> MSGTLVQRLKLILSGGNLRCSDGETACDPERPPTRCVFQVHGQDGSNDTFPLEYVLRLMRSWAHVPCDPYVRVQNTGVSVLFQGFFFRPADAPLAAITAEHNNVILASTHSTGMSLSALDDIKRAGGVDTRPLRAMMSVSCFVRMPRVQLSFRF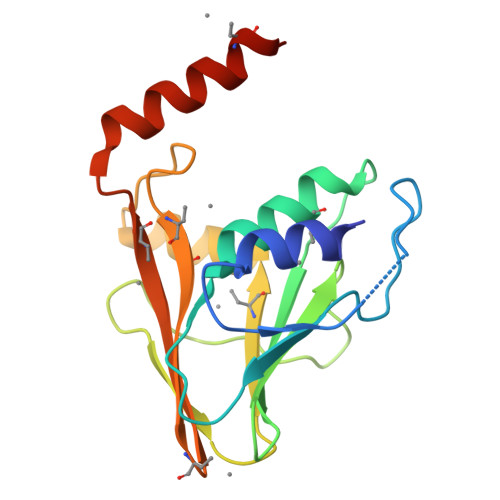MGPDDASQTQRLLDRAEMRQRSVSR>[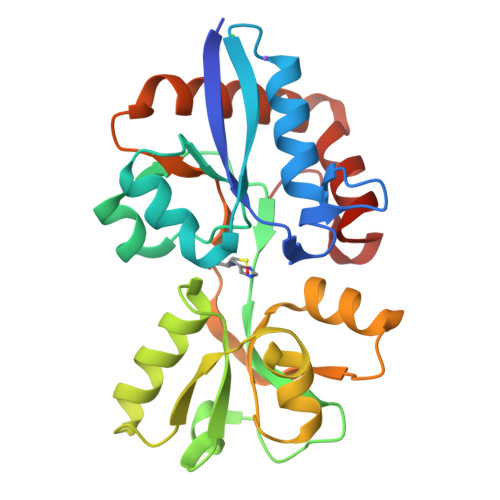2x]SNAANQKVQTITVGTGTQFPNVCFLDENGKLTGYDVELVKEIDKRLPGYKFKFKTMDFSNLLVSLGAGKVDIVAHQMEKSKEREKKFLFNDVAYNNFPLQLTVLDSNNSINSTKDLAGKRVITSATSNGALVLKKINEEQGNNFEIAYEGQGSNDTANQLKTGRADATISTPFAVDFQNKTSAIKEKVVGDVLSNAKVYFMLGKDETKLSKKVDEALQSIIDDGTLKKLSEKWLGADYSKEQY> MKKLSRTISGVTPVAVMTKPLPCPGKCIYCPTFAATPQSYTPESPAVLRAKSCEYQAYKQVALRLRIIQDMGHPTDKVELIIMGGTFLSADITYQYGFIKDCYDALNGVVAGSLEEAKTINETAQHRCVGLCIETRPDICGKAEIQRMIDFGTTRVELGVQMLDDDIYKLVERGHRVSDVAEATCLLREYGLKVHYHWMPGLPGSSPEKDLALSRMVFEDPRFCPDGLKLYPTMVVEGTILEQWWKEGRYTPYPNGTMTGLIADIKALVPPYVRISRVLRDIPAVFISAGLKDSL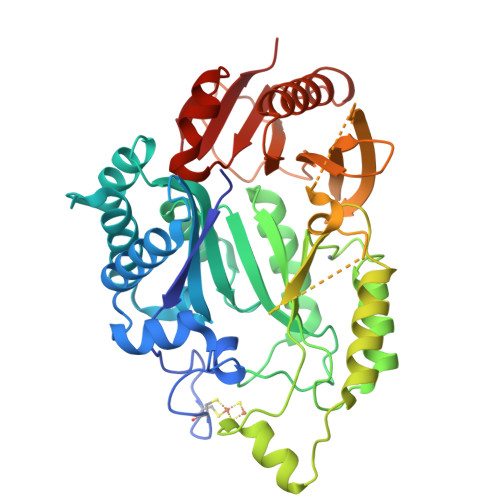RDGVRQILESRHQKCRCIRCREYGHRQRKGQTSGEPTLRRLDYPASGGKEIFLSFEDASDTLYGLLRLRIPCASLPVLGQKYGAKTGLVRELHVGSGSGGLGRKLLAEAECLARDEFGLDSLAILSGVGAREYYRSLGYELVAGYMCKHLD> ESH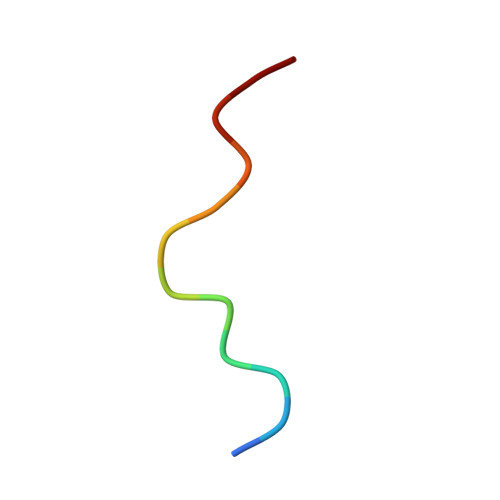PLTVGSLRR> AAQTNAPWGLARISSTSPGTSTYYYDESAGQGSCVYVIDTGIEASHPEFEGRAQMVKTYYYSSRDGNGHGTHCAGTVGSRTYGVAKKTQLFGVKVLDDNGSGQYSTIIAGMDFVASDKNNRNCPKGVVASLSLGGGY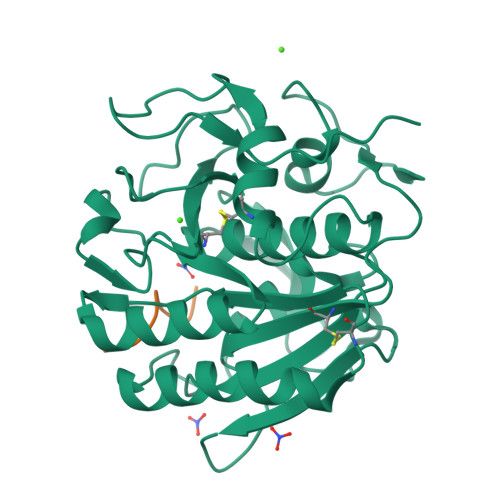SSSVNSAAARLQSSGVMVAVAAGNNNADARNYSPASEPSVCTVGASDRYDRRSSFSNYGSVLDIFGPGTDILSTWIGGSTRSISGTSMATPHVAGLAAYLMTLGKTTAASACRYIADTANKGDLSNIPFGTVNLLAYNNYQA;> PAPFAAA> MATSNLLKNKGSLQFEDKWDFMHPIVLKLLRQESVTKQQWFDLFSDVHAVCLWDDKGSSKIHQALKEDILEFIKQAQARVLSHQDDTALLKAYIVEWRKFFTQCDILPKPFCQLEVTLLGKQSSNKKSNMEDSIVRKLMLDTWNESIFSNIKNRLQDSAMKLVHAERLGEAFDSQLVIGVRESYVNLCSNPEDKLQIYRDNFEKAYLDSTERFYRTQAPSYLQQNGVQNYMKYADAKLKEEEKRALRYLETRRECNSVEALMECCVNALVTSFKETIL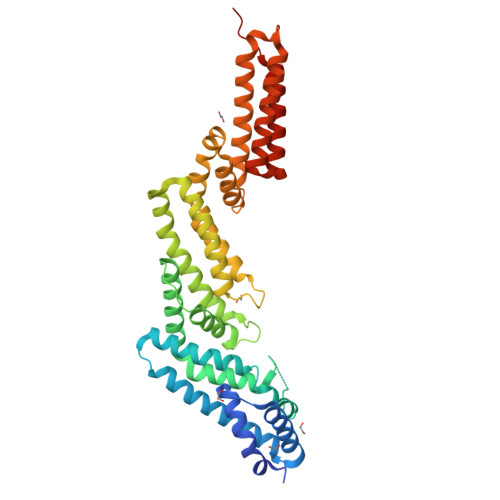AECQGMIKRNETEKLHLMFSLMDKVPNGIEPMLKDLEEHIISAGLADMVAAAETITTDSEKYREQLDTLFNRFSKLVKEAFQDDPRFLTARDKAYKAVVNDATIFKAENLYFQ> DRQQYLRQEVLRRAEATA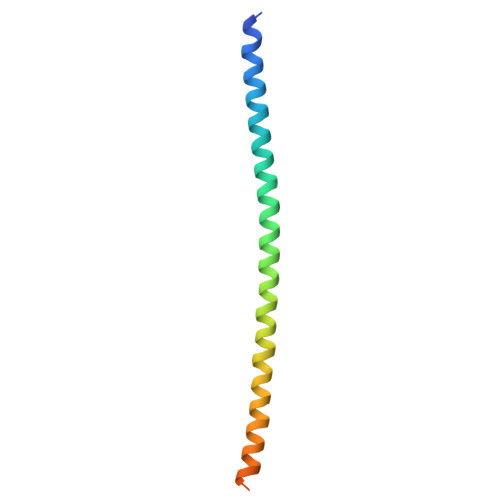ASTSRSLALMYESEKVGVASSEELARQRGVLERTEKMVDKMDQDLKISQKHINSIKSVFGGLVNYFKSKPVET>[7x]GMAEVGEIIEGCRLPVLRRNQDNEDEWPLAEILSVKDISGRK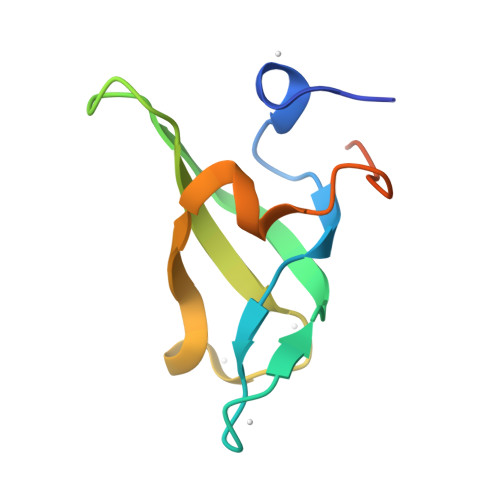LFYVHYIDFNKRLDEWVTHERLDLKKIQFPKKEAKTPTK(5M)-5-(1H-tetrazol-5-yl)-3-[4-(trifluoromethyl)phenyl]-2,1-benzoxazole 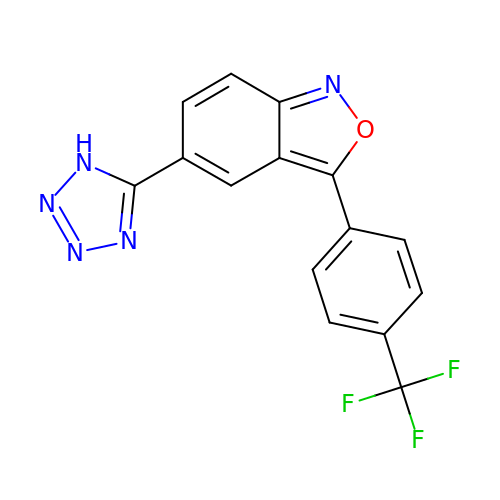| C15 H8 F3 N5 O | JAPDOBATQZBKTD-UHFFFAOYSA-N Here, we report the crystal structures of PhoExo I, which shares 76% amino acid sequence identity with PfuExo I. In this study, we determined three substrate-free structures of PhoExo I and four structures of PhoExo I in complexes with ssDNAs. PhoExo I forms a trimer in solution similar to PfuExo I. The 3′-5′ exonuclease assay of PhoExo I showed that PhoExo I cleaved an ssDNA from its 3′-end at every two nucleotides, and the cleavage stopped at the third to fifth nucleotide from the 5′-end. PhoExo I is predicted to utilize a DEDE (RNase HIII)-type catalytic motif for the hydrolysis of ssDNA. PhoExo I is a novel RNase H superfamily protein.

To examine the mechanisms of ssDNA recognition and cleavage by PhoExo I, we cocrystallized PhoExo I with poly-dA, poly-dC and poly-dT. To prevent the degradation of ssDNA during the cocrystallization, we used the D80N mutant of PhoExo I; the corresponding mutation was previously utilized in a cocrystallization study of the B. halodurans RNase HI―DNA/RNA hybrid complex. In this study, we determined the crystal structures of PhoExo I in complexes with poly-dA, poly-dC and poly-dT at 2.05 Å, 2.50 Å and 2.05 Å, respectively. Each crystal contained one PhoExo I trimer and three oligonucleotides in the asymmetric unit. Although the overall structures of the PhoExo I―ssDNA complexes were nearly identical, PhoExo I formed some base-specific interactions with ssDNAs. In addition, the base groups of the poly-dC and poly-dT formed direct hydrogen bonds with Arg55 and Arg104, and they formed water-mediated hydrogen bonds with Phe17 and Asn214. These interactions may support the substrate recognition of PhoExo I; PhoExo I prefers poly-dT because PhoExo I forms the largest number of base-specific interactions with poly-dT compared to poly-dA and poly-dC. Meanwhile, tracts of adenines are known to exhibit strong base stacking tendencies and increase rigidity of ssDNA. Because the active sites of the PhoExo I trimer are covered by the flexible α2 and α3 helices, it is hard to recruit structurally rigid or partially structured ssDNA to the active sites. PhoExo I may disfavour structurally rigid poly-dA as a substrate. The PhoExo I―ssDNA structures determined in this study are predicted to present the distributive cleavage state of PhoExo I. In this state, PhoExo I recognizes ssDNA only at the active site pocket that accommodates the 3′-OH terminal 4 nt of ssDNA, so the 5′-terminal 3 nt are disordered in the complex structures.

>MRIVAADTGGAVLDESFQPVGLIATVAVLVEKPYKTSKRFLVKYADPYNYDLSGRQAIRDEIELAIELAREVSPDVIHLNSTLGGIEVRKLDESTIDALQISDRGKEIWKELSKDLQPLAKKFWEETGIEIIAIGKSSVPVRIAEIYAGIFSVKWALDNVKEKGGLLVGLPRYMEVEIKKDKIIGKSLDPREGGLYGEVKTEVPQGIKWELYPNPLVRRFMVFEITSKSHHHH[3x]>AAFEAHDYALAERQAQALLAHPATASGARFMLGYVYAFMDRFDEARASFQALQQQAQKSGDHTAEHRALHQVGMVERMAGNWDAARRCFLEERELLASLPEDPLAASANAYEVATVALHFGDLAGARQEYEKSLVYAQQADDQVAIACAF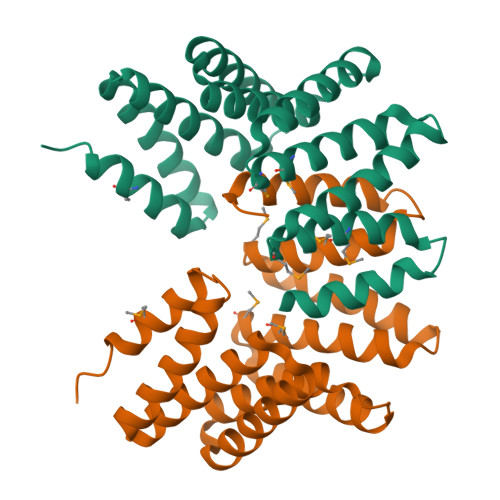RGLGDLAQQEKNLLEAQQHWLRARDIFAELEDSEAVNELMTRLNGLEHHHHHH[2x]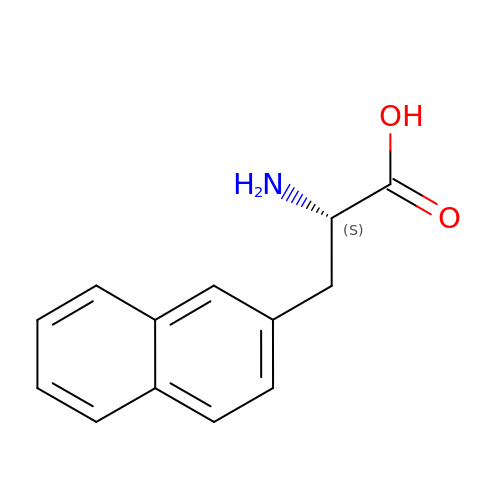BETA-(2-NAPHTHYL)-ALANINE | C13 H13 N O2 | JPZXHKDZASGCLU-LBPRGKRZSA-N The E protein is a class II fusion protein and the largest of the structural proteins. It is the main protein responsible for receptor binding and fusion, as well as the major target for neutralizing antibodies. The prM protein is a precursor that is cleaved by the host cell protease furin into mature M protein and a pr peptide.

Langat virus (LGTV) is a tick isolate with naturally low pathogenicity in mice. It has approximately 85% amino acid identity with TBEV and is often used in research as a biosafety level 2 model virus of more pathogenic tick-borne flaviviruses. We determined the structures of LGTV and chimeric LGTVT:prME using cryogenic electron microscopy (cryo-EM) and three-dimensional image reconstruction. The electron micrographs of virus preparations contained mainly intact spherical virions with a size of ~50 nm in diameter, along with some broken particles. We generated a 3.22 Å resolution map of LGTVT:prME and a 3.82 Å resolution map of LGTV (Fig. 2A through C; Fig. S1A through D). We compared both atomic models to the previously published model of TBEV isolate Kuutsalo-14 (25). The new models included two extra residues in the C-terminus of the E protein (residues 495 and 496), and the LGTVT:prME model has one more residue in the C-terminus of the M protein (residue 75). Both structures are consistent with those of TBEV, with the root mean square deviation (RMSD) of Cα atoms across protein chains below 0.7 Å for the E proteins and below 1.5 Å for the M proteins. When grown in A549 Mavs-/- cells, LGTVT:prME particles contained different glycan structures at this position, identified as complex type (17%), hybrid structures (27%), and oligomannose type (56%). The main complex-type glycan was biantennary digalactosylated with core fucosylation, including GlcNAc with core fucosylation, whereas the LGTV and LGTVT:prME resolve only the innermost GlcNAc of the N-linked glycan at position N154 (Fig. 2F through H).

>SRCTHLENRDFVTGVQGTTRLTLVLELGGCVTVTADGKPSLDVWLDSIYQESPAQTREYCLHAKLTGTKVAARCPTMGPATLPEEHQSGTVCKRDQSDRGWGNHCGLFGKGSIVTCVKFTCEDKKKATGHVYDVNKITYTIKVEPHTGEFVAANETHSGRKSASFTVSSEKTILTLGDYGDVSLLCRVASGVDLAQTVVLALDKTHEHLPTAWQVHRDWFNDLALPWKHDGAEAWNEAGRLVEFGTPHAVKMDVFNLGDQTGVLLKSLAGVPVASIEGTKYHLKSGHVTCEVGLEKLKMKGLTYTVCDKTKFTWKRAPTDSGHDTVVMEVGFSGTRPCRIPVRAVAHGVPEVNVAMLITPNPTMENNGGGFIEMQLPPGDNIIYVGDLNHQWFQKGSSIGRVLQKTRKGIERLTVLGEHAWDFGSVGGVMTSIGRAMHTVLGGAFNTLLGGVGFLPKILLGVAMAWLGLNMRNPTLSMGFLLSGGLVLAMTLGVGA[3x];>[3x]VLIPSHAQRDLTGRGHQWLEGEAVKAHLTRVEGWVWKNKLFTLSLVMVAWLMVDGLLPRILIVVVALALAPAYA>[4x]GSIWDAIAGCEAGGNWAINTGNGYYGGVQFDQGTWEANGGLRYAPRADLAT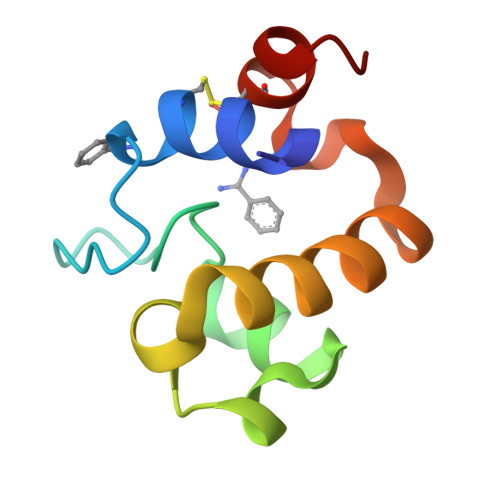REEQIAVAEVTRLRQGWGAWPVCAARAGAR4-CARBOXYPHENYLBORONIC ACID | C7 H7 B O4 | 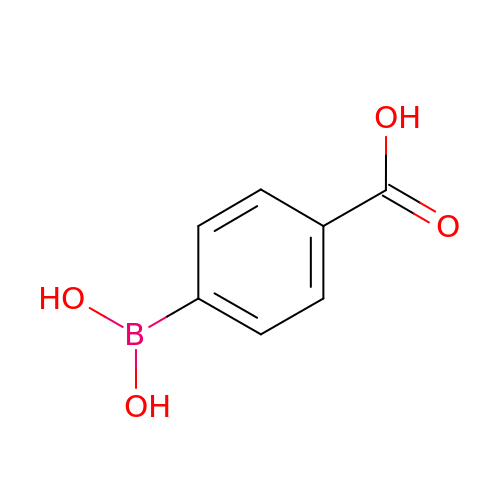SIAVMDKGVRXFAX-UHFFFAOYSA-N>MASMTGGQQMGRIHFHYFKLAVQPQVNKEIRNNNDINIDRTLVAKQSVVKFQLKTADLPAGRDETTSFV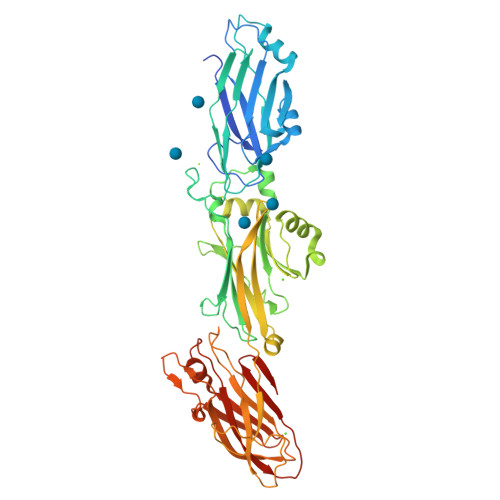LVDPLPSGYQFNPEATKAASPGFDVTYDNATNTVTFKATAATLATFNADLTKSVATIYPTVVGQVLNDGATYKNNFTLTVNDAYGIKSNVVRVTTPGKPNDPDNPNNNYIKPTKVNKNENGVVIDGKTVLAGSTNYYELTWDLDQYKNDRSSADTIQKGFYYVDDYPEEALELRQDLVKITDANGNEVTGVSVDNYTNLEAAPQEIRDVLSKAGIRPKGAFQIFRADNPREFYDTYVKTGIDLKIVSPMVVKKQMGQTGGSYENQAYQIDFGNGYASNIVINNVPKINPKKDVTLTLDPADTNNVDGQTIPLNTVFNYRLIGGIIPANHSEELFKYNFYDDYDQTGDHYTGQYKVFAKVDITLKNGVIIKSGTELTQYTTAEVDTTKGAITIKFKEAFLRSVSIDSAFQAESYIQMKRIAVGTFENTYINTVNGVTYSSLEHHHHHH[2x]> GSDLPAGWMRVQDTSGTYYWHIPTGTTQWEPPGR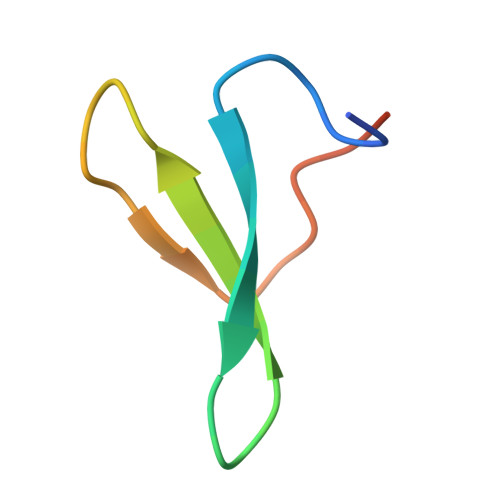ASPS>SMKVTKVGGISHKKYTSEGRLVKSESEENRTDERLSALLNMRLDMYIKNPSSTETKENQKRIGKLKKFFSNKMVYLKDNTLSLKNGKKENIDREYSETDILESDVRDKKNFAVLKKIYLNENVNSEELEVFRNDIKKKLNKINSLKYSFEKNKANYQKINENNIEKVEGKSKRNIIYDYYRESAKRDAYVSNVKEAFDKLYKEEDIAKLVLEIENLTKLEKYKIREFYHEIIGRKNDKENFAKIIYEEIQNVNNMKELIEKVPDMSELKKSQVFYKYYLDKEELNDKNIKYAFCHFVEIEMSQLLKNYVYKRLSNISNDKIKRIFEYQNLKKLIENKLLNKLDTYVRNCGKYNYYLQDGEIATSDFIARNRQNEAFLRNIIGVSSVAYFSLRNILETENENDITGRMRGKTVKNNKGEEKYVSGEVDKIYNENKKNEVKENLKMFYSYDFNMDNKNEIEDFFANIDEAISSIRHGIVHFNLELEGKDIFAFKNIAPSEISKKMFQNEINEKKLKLKIFRQLNSANVFRYLEKYKILNYLKRTRFEFVNKNIPFVPSFTKLYSRIDDLKNSLGIYWKTPKTNDDNKTKEIIDAQIYLLKNIYYGEFLNYFMSNNGNFFEISKEIIELNKNDKRNLKTGFYKLQKFEDIQEKIPKEYLANIQSLYMINAGNQDEEEKDTYIDFIQKIFLKGFMTYLANNGRLSLIYIGSDEETNTSLAEKKQEFDKFLKKYEQNNNIKIPYEINEFLREIKLGNILKYTERLNMFYLILKLLNHKELTNLKGSLEKYQSANKEEAFSDQLELINLLNLDNNRVTEDFELEADEIGKFLDFNGNKVKDNKELKKFDTNKIYFDGENIIKHRAFYNIKKYGMLNLLEKIADKAGYKISIEELKKYSNKKNEIEKNHKMQENLHRKYARPRKDEKFTDEDYESYKQAIENIEEYTHLKNKVEFNELNLLQGLLLRILHRLVGYTSIWERDLRFRLKGEFPENQYIEEIFNFENK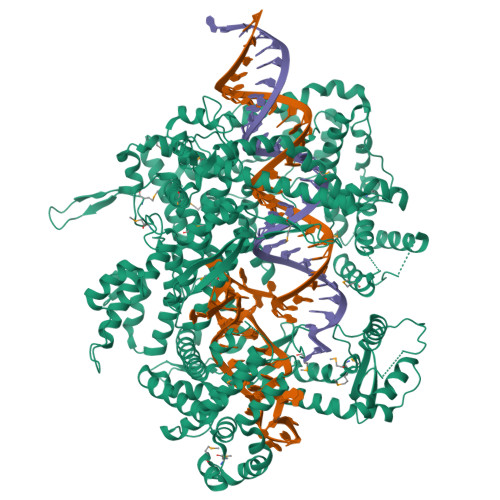KNVKYKGGQIVEKYIKFYKELHQNDEVKINKYSSANIKVLKQEKKDLYIANYIAAFNYIPHAEISLLEVLENLRKLLSYDRKLKNAVMKSVVDILKEYGFVATFKIGADKKIGIQTLESEKIVHLKNLKKKKLMTDRNSEELCKLVKIMFEYKMEEKKSEN[2x]4-methyl-3-[(2-pyridin-3-ylquinazolin-4-yl)amino]-~{N}-[3-(trifluoromethyl)phenyl]benzamide | C28 H20 F3 N5 O | 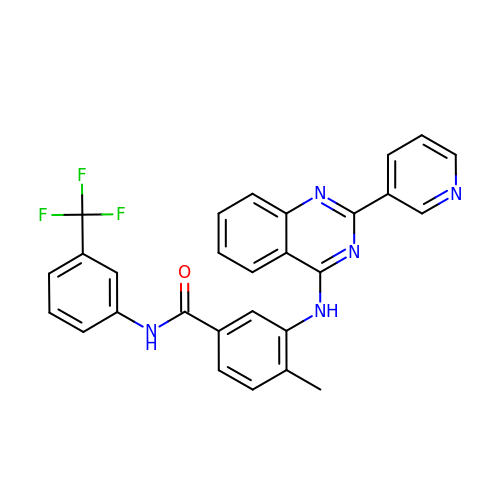IGEHRXWXMHBWMM-UHFFFAOYSA-N> MHHHHHHHAVRASEISRVYEAYPEKKATLYFLVLGFLALIVGSLFGPFQALNYGNVDAYPLLKRLLPFVQSYYQGLTLHGVLNAIVFTQLFAQAIMVYLPARELNMRPNMGLMWLSWWMAFIGLVVFALPLLANEATVLYTFYPPLKGHWAFYLGASVFVLSTWVSIYIVLDLWRRWKAANPGKVTPLVTYMAVVFWLMWFLASLGLVLEAVLFLLPWSFGLVEGVDPLVARTLFWWTGHPIIYFWLLPAYAIIYTILPKQAGGKLVSDPMARLAFLLFLLLSTPVGFHHQFADPGIDPTWKMIHSVLTLFVAVPSLMTAFTVAASLEFAGRLRGGRGLFGWIRALPWDNPAFVAPVLGLLGFIPGGAGGIVNASFTLDYVVHNTAWVPGHFHLQVASLVTLTAMGSLYWLLPNLTGKPISDAQRRLGLAVVWLWFLGMMIMAVGLHWAGLLNVPRRAYIAQVPDAYPHAAVPMVFNVLAGIVLLVALLLFIYGLFSVLLSRERKPELAEAPLPFAEVISGPEDRR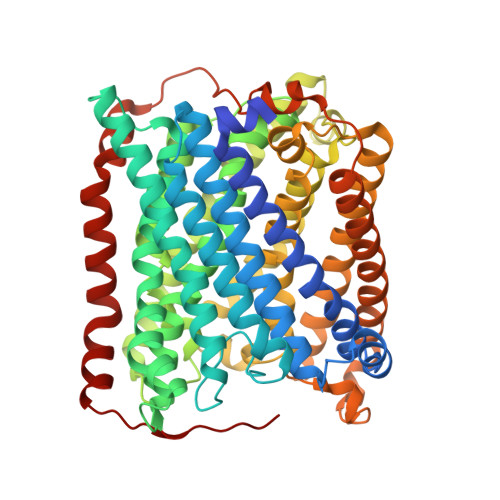LVLAMDRIGFWFAVAAILVVLAYGPTLVQLFGHLNPVPGWRLW>[2x]GASLEHHHHHHENLYFQSGTRWAVLVAGSSGYWNYRHQADICHAYQLLRKG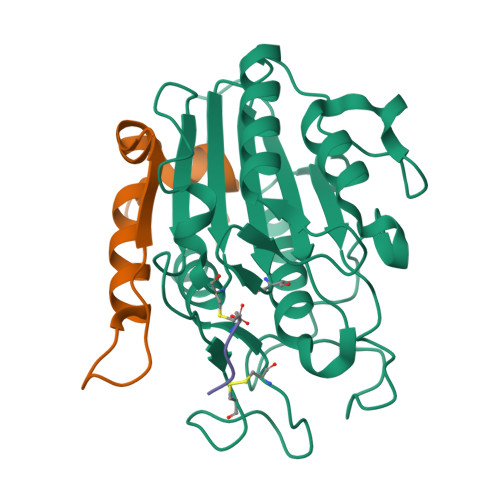GLKEENIVVFMYDDIANNYENPRPGTIINSPHGKDVYQGVPKDYTGDDVNVDNLFAVILGDKTAVKGGSGKVVDSGPNDHIFIFYSNHGGPGVLGMPTSPYLYANDLNDVLKKKHALGTYKSLVFYLEACESGSIFEGLLPEGLNIYATTASNAEESSWGTYCPGEEPSPPPEYETCLGDLYSVAWMEDSGMHN;>[2x]LQTETLHQQYELVKRRTAPVGYSYGSHVMQYGDVGISKDNLDLYMGTNPAN> LVPRGSHMKDDYSSSLSNNNLGWTDPTEFPLGCSPNVTTPKNGLSMELYSYDYLKSGSNPCWDAAYLDPNYPRTGYKSHRLLAKVENVAGNINFYYHAPMGCTSLFDTLPQAYNYRTPLTMTNFTMLLYGYFKPKVTGYHTFTISADDLLFVNFGAGNAFDCCKRESSADDFGNYQAYAVWGSQTAKDDLTVHLDAGLYYPIRIFFNNRDNDGALSLTLKTESDPNPVIDFSDYFYSFDDTKDGCPGLVSYD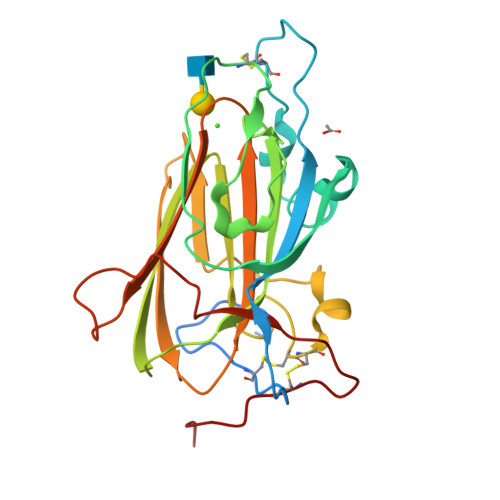TS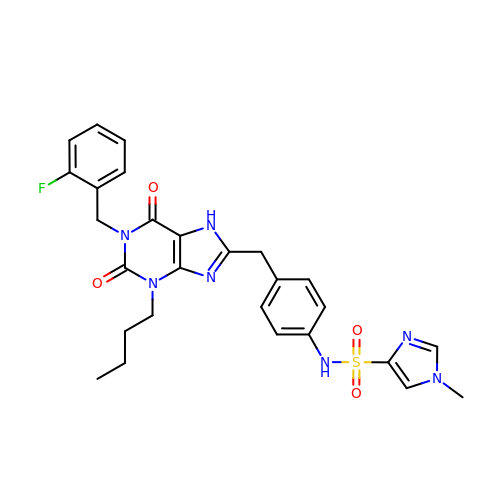N-(4-{[3-BUTYL-1-(2-FLUOROBENZYL)-2,6-DIOXO-2,3,6,7-TETRAHYDRO-1H-PURIN-8-YL]METHYL}PHENYL)-1-METHYL-1H-IMIDAZOLE-4-SULFONAMIDE | C27 H28 F N7 O4 S | OWJCXBGUTOMZTE-UHFFFAOYSA-N>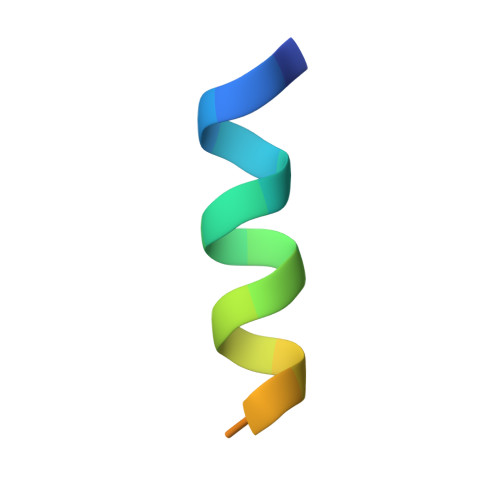 DDDIVFEDFARQRLKGMKDD Cholesterol oxidase (COx) (E.C 1.1.3.6) is a flavoenzyme catalysing the oxidation and isomerisation of cholesterol through a hydride transfer mechanism from the substrate to the FAD reactive center (N5) resulting in reduction of the FAD cofactor. The Type I COx is a member of the Glucose-Methanol-Choline (GMC) oxidoreductase family, members of which share a similar active site architecture despite catalysing different biochemical reactions. Density functional theory calculations also carried out as part of this study suggest that a conserved hydrogen bond from the main chain nitrogen atom of Gly120 to the FAD-N5 atom facilitates hydride transfer by re-arrangement of the lone pair of electrons on N5. One subset of flavoenzymes are the oxidoreductases which catalyse the dehydrogenation of their substrate and require oxygen for reoxidizing the reduced flavin cofactor.

Therefore, to further investigate the role of hydrogen atoms in stabilization of the flavin cofactor during redox catalysis by COx we have determined the neutron structure of a H/D-exchanged crystal of COx (H/D-COx) to 2.2 Å resolution. A single H/D-exchanged crystal of COx was used to collect both neutron and X-ray diffraction data and joint X-ray and neutron refinement of the H/D-COx structure was carried out to 2.2 Å resolution. No significant structural differences were found between the current X-ray/Neutron structure and previously determined X-ray structures of COx. Two deuterium atoms, one involved in a conserved hydrogen bond between Gly120-NH and FAD-N5 and one involved in a hydrogen bond between the conserved water molecule, Wat541, and the proposed base (Glu361) in the substrate oxidation reaction, were clearly observed in the nuclear difference density maps and provide insight into both substrate binding and hydride transfer events in COx. The neutron structure of COx reveals an intriguing conserved interaction between the amide nitrogen atom of Gly120 and N5 of the FAD cofactor resulting in an elongated main chain N-H bond length. Modeling this scenario with partial occupancies of H/D also confirmed highly occupied deuterium and resulted in residual density between the modeled H/D positions. These observations indicating the nuclear density is the result of an elongated N-D bond rather than an average of partially occupied deuterium atoms on both Gly120 and FAD-N5. The three deuterium atoms of the Lys225 side chain are clearly visible in the nuclear density maps indicating that this group has a positive charge and that the ammonium group of the side chain is statically positioned in the structure due to the interaction with the carbonyl oxygen atom of the peptide bond between Asn119 and Gly120.

> DNGGYVPAVVIGTGYGAAVSALRLGEAGVQTLMLEMGQLWNQPGPDGNIFCGMLNPDKRSSWFKNRTEAPLGSFLWLDVVNRNIDPYAGVLDRVNYDQMSVYVGRGVGGGSLVNGGMAVEPKRSYFEEILPRVDSSEMYDRYFPRANSMLRVNHIDTKWFEDTEWYKFARVSREQAGKAGLGTVFVPNVYDFGYMQREAAGEVPKSALATEVIYGNNHGKQSLDKTYLAAALGTGKVTIQTLHQVKTIRQTKDGGYALTVEQKDTDGKLLATKEISCRYLFLGAGSLGSTELLVRARDTGTLPNLNSEVGAGWGPNGNIMTARANHMWNPTGAHQSSIPALGIDAWDNSDSSVFAEIAPMPAGLETWVSLYLAITKNPQRGTFVYDAATDRAKLNWTRDQNAPAVNAAKALFDRINKANGTIYRYDLFGTQLKAFADDFCYHPLGGCVLGKATDDYGRVAGYKNLYVTDGSLIPGSVGVNPFVTITALAERNVERIIKQDVTASHHHHHH> GPLGSPEFPGSDRNSVDYAQIASGID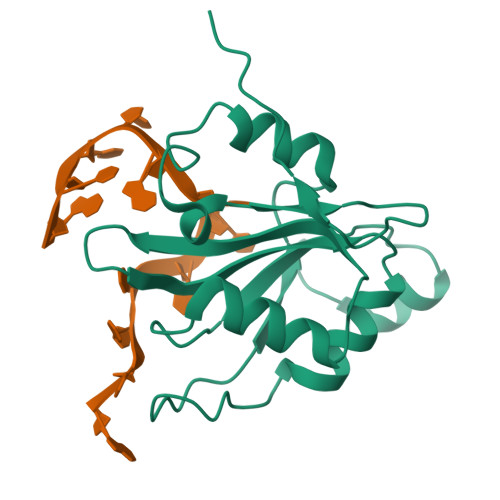TRTTVMIKNIPNKFTQQMLRDYIDVTNKGTYDFLYLRIDFVNKCNVGYAFINFIEPQSIITFGKARVGTQWNVFHSEKICDISYANIQGKDRLIEKFRNSCVMDENPAYRPKIFVSHGPNRGMEEPFPAPNNARRKLRSIASAQQIGLFPPTASKC>VNRLDAIVWENIEGNLSRAFLTLDLHAFFNVNKEVGDGNCFYRALSRLHSESRTSNEHLYYRLLIPDAVDKYFDIEPEAIGLGLNKQEYVSKAILDGEWAGSLEASMLSKFLDITIIIWIVDDSGTIISANRYGEGRPSQAYNLCMVGNAHFDSLYIRV[2x];>[2x]PLSILVRNERGHSNIYEVFLTQTVDTLKKKVSQR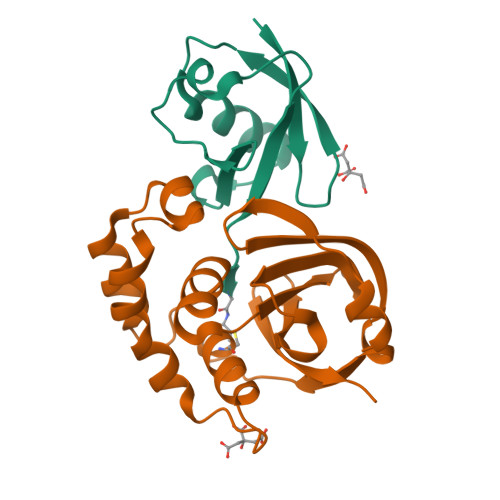EQVHEDQFWLSFEGRPMEDKELLGEYGLKPQCTVIKHLRLRG> GSHMASMKKKGSVVIVGRINLSGDTAYAQQTRGEEGCQETSQTGRDKNQVEGEVQIVSTATQTFLATSINGVLWTVYHGAGT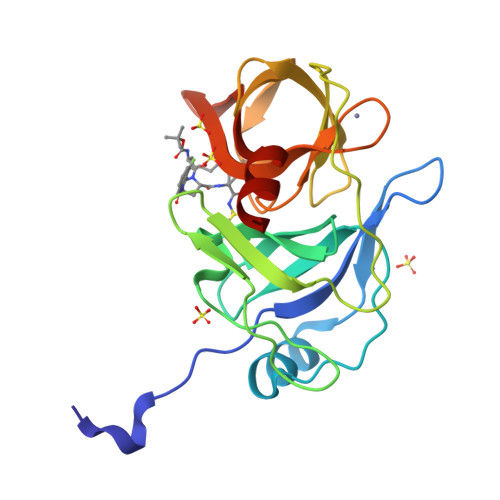RTIASPKGPVTQMYTNVDKDLVGWQAPQGSRSLTPCTCGSSDLYLVTRHADVIPVRRRGDSRGSLLSPRPISYLKGSAGGPLLCPAGHAVGIFRAAVSTRGVAKAVAFIPVESLETTMRSP>MQKQRTTSQWRELDAAHHLHPFTDTASLNQAGARVMTRGEGVYLWDSEGNKIIDGMAGLWCVNVGYGRKDFAEAARRQMEELPFYNTFFKTTHPAVVELSSLLAEVTPAGFDRVFYTNSGSESVDTMIRMVRRYWDVQGKPEKKTLIGRWNGYHGSTIGGASLGGMKYMHEQGDLPIPGMAHIEQPWWYKHGKDMTPDEFGVVAARWLEEKILEIGADKVAAFVGEPIQGAGGVIVPPATYWPEIERICRKYDVLLVADEVICGFGRTGEWFGHQHFGFQPDLFTAA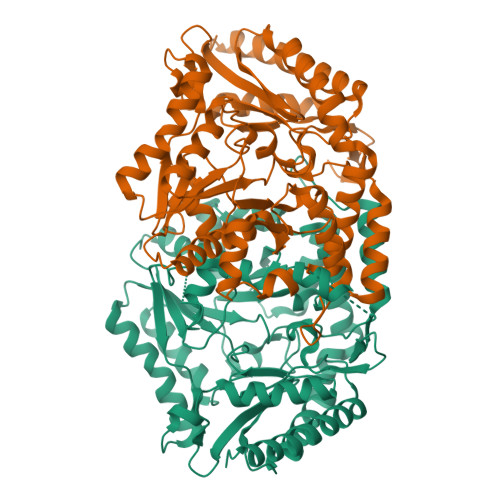KGLSSGYLPIGAVFVGKRVAEGLIAGGDFNHGFTYSGHPVCAAVAHANVAALRDEGIVQRVKDDIGPYMQKRWRETFSRFEHVDDVRGVGMVQAFTLVKNKAKRELFPDFGEIGTLCRDIFFRNNLIMRACGDHIVSAPPLVMTRAEVDEMLAVAERCLEEFEQTLKARGLA[4x]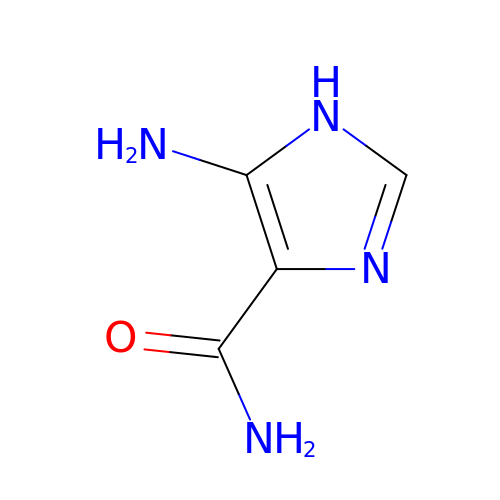5-amino-1H-imidazole-4-carboxamide | C4 H6 N4 O | DVNYTAVYBRSTGK-UHFFFAOYSA-N> ASPQVSVTLQLVVDSSMFAKYNGDAKKIVTVLDTRVNIMKSIFKPLLLLITLSGIEMWTSKDLIT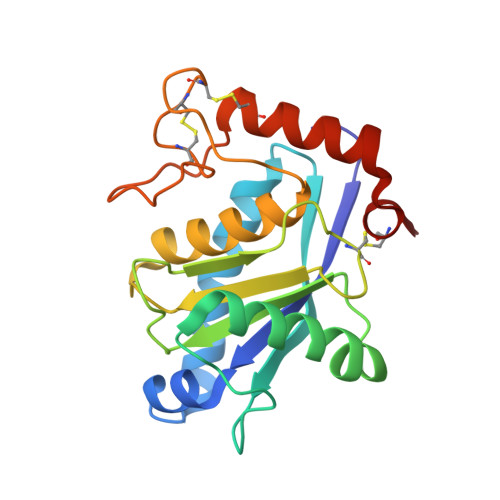VKPAGDLTLSLFADWRQTLLLSRILNDNAQLQTAVDFRGAVVGLAFVGTMCNAKYSAGIIQDFSAIPLLMAVVMAHELGHNLGMLHDDGYSCDCDVCIMAPSLSSDPTKVFSNCSLILYEDFLSNEEPDCIDNASNN>[6x]MCWAAAIPIAISGAQAISGQNAQAKMIAAQTAAGRRQAMEIMRQTNIQNADLSLQARSKLEEASAELTSQNMQKVQAIGSIRAAIGESMLEGSSMDRIKRVTEGQFIREANMVTENYRRDYQAIFAQQLGGTQSAASQIDEIYKSEQKQKSKLQMVLDPLAIMGSSAASAYASGAFDSKSTTKAPIVAAKGTKTGR;>[12x]MCFSPKIKTPKMDTNQIRAVEPAPLTQEVSSVEFGGSSDETDTEGTEVSGRKGLKVERDDSVAKSKASGNGSARMKSSIRKSAFGGKK;>[12x]MAEKRTGLAEDGAKSVYERLKNDRAPYETRAQNCAQYTIPSLFPKDSDNASTDYQTPWQAVGARGLNNLASKLMLALFPMQTWMRLTISEYEAKQLLSDPDGLAKVDEGLSMVERIIMNYIESNSYRVTLFEALKQLVVAGNVLLYLPEPEGSNYNPMKLYRLSSYVVQRDAFGNVLQMVTRDQIAFGALPEDIRKAVEGQGGEKKADETIDVYTHIYLDEDSGEYLRYEEVEGMEVQGSDGTYPKEACPYIPIRMVRLDGESYGRSYIEEYLGDLRSLENLQEAIVKMSMISSKVIGLVNPAGITQPRRLTKAQTGDFVTGRPEDISFLQLEKQADFTVAKAVSDAIEARLSFAFMLNSAVQRTGERVTAEEIRYVASELEDTLGGVYSILSQELQLPLVRVLLKQLQATQQIPELPKEAVEPTISTGLEAIGRGQDLDKLERCVTAWAALAPMRDDPDINLAMIKLRIANAIGIDTSGILLTEEQKQQKMAQQSMQMGMDNGAAALAQGMAAQATASPEAMAAAADSVGLQPGI;>MRSYDMNVETAAELSAVNDILASIGEPPVSTLEGDANADAANARRILNKINRQIQSRGWTFNIEEGITLLPDVYSNLIVYSD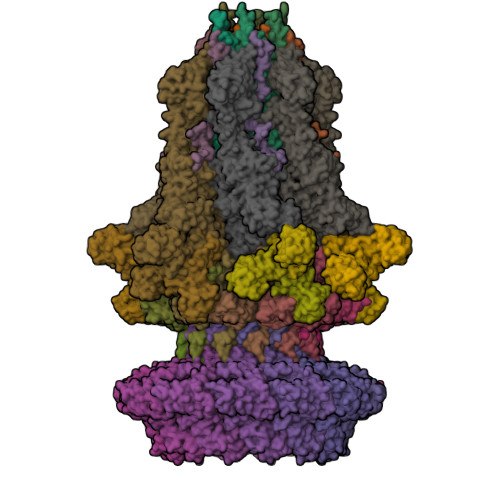DYLSLMSTSGQSIYVNRGGYVYDRTSQSDRFDSGITVNIIRLRDYDEMPECFRYWIVTKASRQFNNRFFGAPEVEGVLQEEEDEARRLCMEYEMDYGGYNMLDGDAFTSGLLTR[12x];>[18x]MANVIKTVLTYQLDGSNRDFNIPFEYLARKFVVVTLIGVDRKVLTINTDYRFATRTTISLTKAWGPADGYTTIELRRVTSTTDRLVDFTDGSILRAYDLNVAQIQTMHVAEEARDLTTDTIGVNNDGHLDARGRRIVNLANAVDDRDAVPFGQLKTMNQNSWQARNEALQFRNEAETFRNQAEGFKNESSTNATNTKQWRDETKGFRDEAKRFKNTAGQYATSAGNSASAAHQSEVNAENSATASANSAHLAEQQADRAEREADKLENYNGLAGAIDKVDGTNVYWKGNIHANGRLYMTTNGFDCGQYQQFFGGVTNRYSVMEWGDENGWLMYVQRREWTTAIGGNIQLVVNGQIITQGGAMTGQLKLQNGHVLQLESASDKAHYILSKDGNRNNWYIGRGSDNNNDCTFHSYVHGTTLTLKQDYAVVNKHFHVGQAVVATDGNIQGTKWGGKWLDAYLRDSFVAKSKAWTQVWSGSAGGGVSVTVSQDLRFRNIWIKCANNSWNFFRTGPDGIYFIASDGGWLRFQIHSNGLGFKNIADSRSVPNAIMVENE;>MALISQSIKNLKGGISQQPDILRYPDQGSRQVNGWSSETEGLQKRPPLVFLNTLGDNGALGQAPYIHLINRDEHEQYYAVFTGSGIRVFDLSGNEKQVRYPNGSNYIKTANPRNDLRMVTVADYTFIVNRNVVAQKNTKSVNLPNYNPNQDGLINVRGGQYGRELIVHINGKDVAKYKIPDGSQPEHVNNTDAQWLAEELAKQMRTNLSDWTVNVGQGFIHVTAPSGQQIDSFTTKDGYADQLINPVTHYAQSFSKLPPNAPNGYMVKIVGDASKSADQYYVRYDAERKVWTETLGWNTEDQVLWETMPHALVRAADGNFDFKWLEWSPKSCGDVDTNPWPSFVGSSINDVFFFRNRLGFLSGENIILSRTAKYFNFYPASIANLSDDDPIDVAVSTNRIAILKYAVPFSEELLIWSDEAQFVLTASGTLTSKSVELNLTTQFDVQDRARPFGIGRNVYFASPRSSFTSIHRYYAVQDVSSVKNAEDITSHVPNYIPNGVFSICGSGTENFCSVLSHGDPSKIFMYKFLYLNEELRQQSWSHWDFGENVQVLACQSISSDMYVILRNEFNTFLARISFTKNAIDLQGEPYRAFMDMKIRYTIPSGTYNDDTFTTSIHIPTIYGANFGRGKITVLEPDGKITVFEQPTAGWNSDPWLRLSGNLEGRMVYIGFNINFVYEFSKFLIKQTADDGSTSTEDIGRLQLRRAWVNYENSGTFDIYVENQSSNWKYTMAGARLGSNTLRAGRLNLGTGQYRFPVVGNAKFNTVYILSDETTPLNIIGCGWEGNYLRRSSGI[6x]>GSGGSGKVVKFSYMWTINNFSFCREEMGEVIKSSTFSSGANDKLKWCLRVNPKGLDEESKDYLSLYLLLVSCPKSEVRAKFKFSILNAKGEETKAMESQRAYRFVQGKDWGFKKFIRRDFLLDEANGLLPDDKLTLFCEVSVVQD[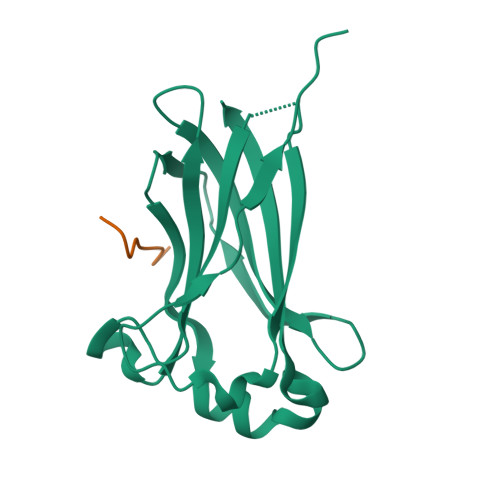2x];>NTLFPDVSSSTH[2x]>[2x]MSYQSTIVPVELHSFEDAQVIGGAFRDGDAVVFDMSLLSREEARRIVDFAAGLCFALR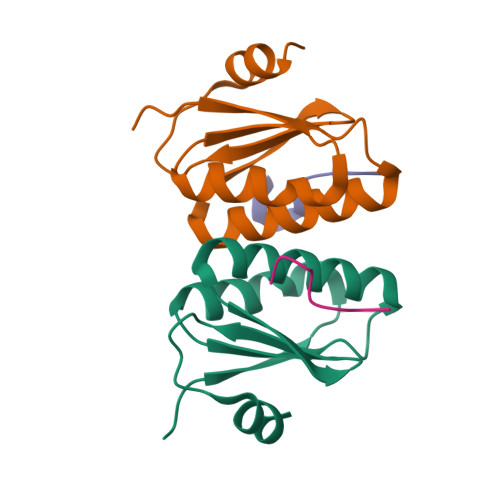GKMQKIDSVTFAVVPELSNISTSELERAARIR;>DDLDVPSFLQ[2x]>NEAVKTLDGWFCLHDFRSIDWAAWRELNPGNQELMLNELSHFLSDMEITKNIGEGEHTIYSILGQKADLVFFTLRDSLEALNEVENRFNKLAIADYLLPTYSYISVVELSNYLASHMAGGDDPYQNKGVRARLYPALPPKKHICFYPMSKKRDGADNWYMLPMEERQQLIRDHGLIGRSYAGKVQQIIGGSIGFDDY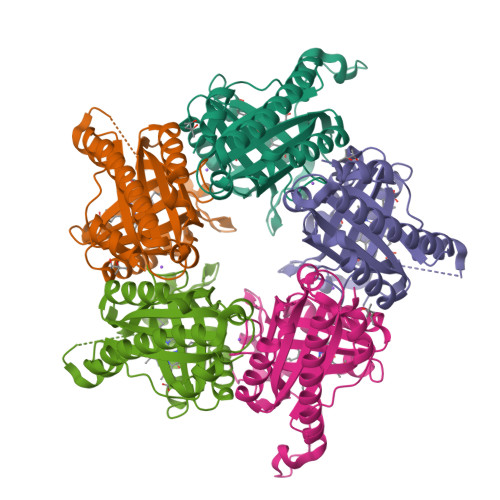EWGVTLFSDDALEFKRIVTEMRFDEASARYAEFGSFFIGNLLLSEQLSKLFTI[5x]>MGNILLRLIVFALDPLGLGRRFLIRPAVNLGWNVYDRVRSKADEKVGTVRELVLRLGLIAFAVVLIIWLAVFMYAAFYYVYMPAISHTRPVHMQFKTCLETSTPCTFPHAHVSL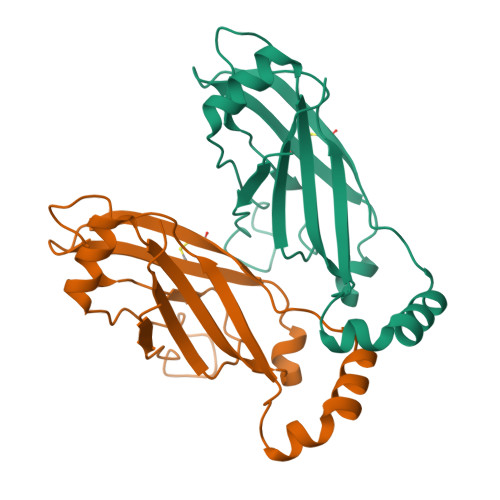TKKQQLLMVGQAYKVIVNIDMPESPQNLELGMFMVCAEMRDYDSMLRGHSCRSAMMRYRSPLIRMISTWVLSPLYVLGWKEEFQQVPVEIFSRYLEERQHPITDVYVEIQSQKIQFYTVTLHIVADFTGLRYIMFNWPVLSAIVAISTNLFFILVVFLLSWYHWSDAKWLHSVQIKYARLTKSLEPGVIHSKASSLRDDDDDLVAYSDKSDIADVGGDTLSDVDADDLVLVKKSRSGKRESPDALRKRPTKKTTADHAAALEHHHHHH[2x]Leukotriene (LT) C4 synthase (LTC4S) catalyzes the conjugation of the fatty acid LTA4 with the tripeptide GSH to produce LTC4, the parent compound of the cysteinyl leukotrienes, important mediators of asthma. LTC4S is a trimeric integral membrane protein and a member of the MAPEG (membrane-associated proteins in eicosanoid and glutathione metabolism) family, which also includes three microsomal GSH S-transferases, 5-lipoxygenase activating protein, and microsomal prostaglandin E synthase 1 (9, 10). The crystal structure of human LTC4S has been solved and identified a unique horseshoe-shaped conformation of GSH bound at the active site by residues from two neighboring monomers. It was postulated that the lipid substrate LTA4 binds in a hydrophobic crevice between two monomers and that Trp-116 could act as a “molecular ruler” for binding of LTA4 with its ω-end buried under the aromatic side chain.

To get a better picture of how the substrate and product bind at the active site and probe the role of Trp-116, we synthesized three mimics of an LTA4-GSH adduct, termed analogs I–III. We solved the structures of wt LTC4S in complex with analogs I, II, and III to 2.75, 3.2, and 2.9 Å. The phenyl ring in analogs II and III were added to increase the visibility of the acyl chain that was to some extent disordered in the analog I complex structure, as well as to stabilize its interactions between the protein and the acyl/phenyl moiety via π-stacking to Trp-116. Analog II showed a higher than expected IC50 value (>10 mm). The binding conformation, however, remains the same for all three analogs. Examination of the active sites in the five analog complex structures reveals a shift in the binding configuration of the GSH part that is similar for all three analogs. The corresponding distance in the structures with analogs I–III is ∼7.8 Å.

> MHHHHHHKDEVALLAAVTLLGVLLQAYFSLQVISARRAFRVSPPLTTGPPEFERVYRAQVNCSEYFPLFLATLWVAGIFFHEGAAALCGLVYLFARLRYFQGYARSAQLRLAPLYASARALWLLVALAALGLLAHFLPAALRAALLGRLRTLLPWA> MAIGLKAYPELCHGCGNCVIACPVNALRSPEVAGGKGPTDDVEIIMIVEDGVVNIKNPDLCGKCGTCVES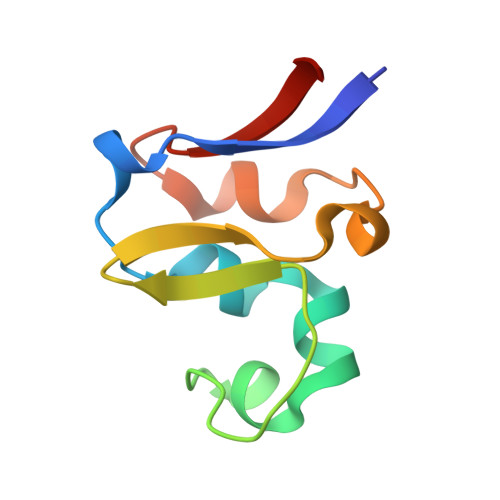CPVDAIRLEELE> SNAMAGNFLENNTVTLVGKVFTPLEFSHELYGEKFFNFILEVPRLS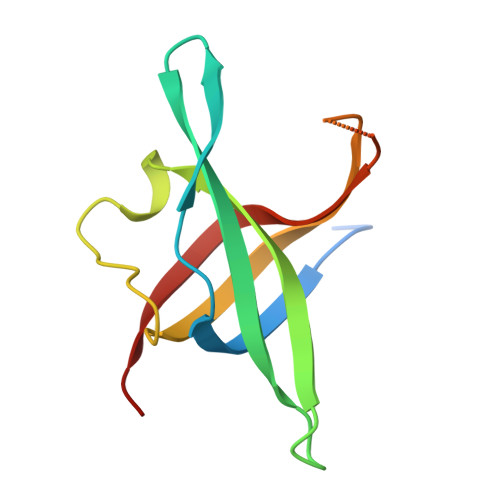ETKDYLPITISNRLFEGMNLEVGTRVKIEGQLRSYNRKSPEEGKNKLILTVFARDISVVPE>APVWGCASTRGRSAEMEDASAAVPRFADVPVRLLASRRDLDALGLDADALR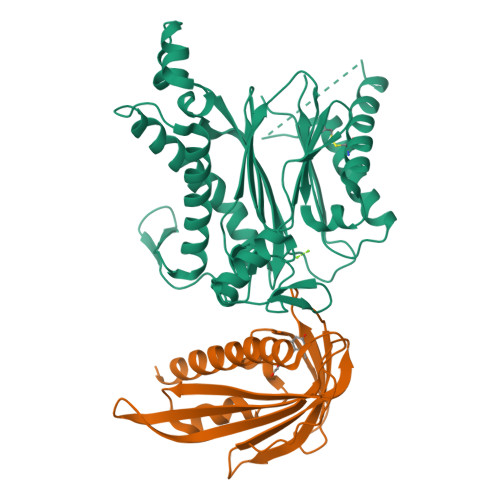LPAHLFGVFDGHGGAEVANYCRERIHVVLSAALARLGKNLGEMGEVDMKEHWDDVFTKCFQRVDDEVSGRVTRVVNGGGEVRSEPVTAENVGSTAVVALVCSSHVVVANCGDSRIVLCRGKEPVALSIDHKPDRKDERARIEAQGGKVIQWNGYRVSGLLAMSRSIGDRYLKPFVIPKPEVMVVPRAKDDDCLILASDGLWDVVSNEEACKVARRQILLWHKNNGAASPLSDEGEGSTDPAAQAAADYLMRLALKKGSEDNITVIVVDLKPRKKLKN[2x];>[2x]ETEYVRRFHRHEPRDHQCSSAVAKHIKAPVHLVWSLVRRFDQPQLFKPFVSRCEMKGNIEIGSVREVNVKSGLPATRSTERLELLDDNEHILSVRFVGGDHRLKNYSSILTVHPEVIDGRPGTLVIESFVVDVPEGNTKDETCYFVEALLKCNLKSLAEVSERLVVKDQTEPLDR2-propenyl-N-acetyl-neuraminic acid | C14 H23 N O8 | 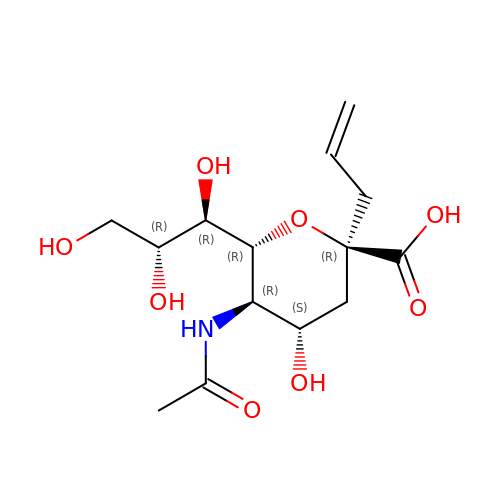IUGVDRFIVSPVGO-KXEMTNKZSA-N> M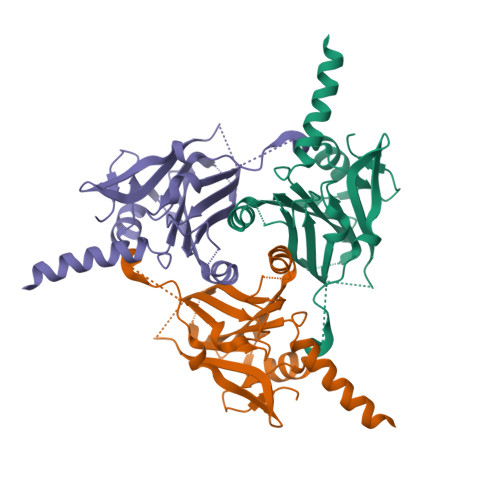ADVAGTSNRDFRGYILSVQAEEQKNYNNSLNGEVSVWVYAYYSDGSVLVINKNSQYKVGISETFKALKEYREGQHNDSYDEYEVNQSIYYPNGGDARKFHSNAKPRAIQIIFSPSVNVRTIKMAKGNAVSVPDEYLQRSHPWEATGIKYKKIKRDGEIVGYSHYFELPHEYNSISLAVSGVHKNPSSYNVGSAHNVMDVFQSCDLALRFCNRYWAELELVNHYISPNAYPYLDINNHSYGVALSNRQ> LLVPKLTASVTDGAVGVTVDAPVSVTAADGVLAAVTMVNDNGRPVAGRLSPDGLRWSTTEQLGYNRRYTLNATALGLGGAATRQLTFQTSSPAHLTMPYVMPGDGEVVGVGEPVAIRFDENIADRGAAEKAIKITTNPPVEGAFYWLNNREVRWRPEHFWKPGTAVDVAVNTYGVDLGEGMFGEDNVQTHFTIGDEVIATADDNTKILTVRVNGEVVKSMPTSMGKDSTPTANGIYIVGSRYKHIIMDSSTYGVPVNSPNGYRTDVDWATQISYSGVFVHSAPWSVGAQGHTNTSHGCLNVSPSNAQWFYDH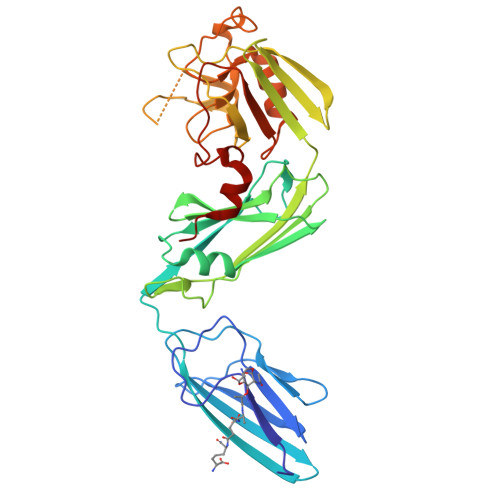VKRGDIVEVVNTVGGTLPGIDGLGDWNIPWDQWRAGNAKA The bifunctional enzyme proline utilization A (PutA) catalyzes the two-step oxidation of L-proline to L-glutamate using proline dehydrogenase (PRODH) and L-glutamate-γ-semialdehyde dehydrogenase (GSALDH) domains. The two active sites are 42 Å apart and connected by a buried tunnel that is hypothesized to channel the intermediates Δ1-pyrroline-5-carboxylate (P5C) and/or L-glutamate-γ-semialdehyde (GSAL). The PRODH active site is located in a (βα)8 barrel, while the GSALDH module features Rossmann NAD+-binding and catalytic domains, which are both characteristic of the ALDH superfamily. Kinetic and conventional X-ray crystallography of PutA from Sinorhizobium meliloti (SmPutA) were used to capture high resolution (1.47–1.88 Å) structures of states along the catalytic cycle, including a novel FADH−-proline covalent adduct in the PRODH site, the intermediate P5C bound noncovalently in the reduced PRODH active site, the covalent acyl-enzyme intermediate of the GSALDH reaction, and noncovalent complexes of GSAL and the final product L-glutamate in the GSALDH active site.

The structure of SmPutA complexed with the product L-glutamate was determined at 1.50 Å resolution. The complex was prepared by soaking WT crystals with 325 mM L-glutamate. Electron density for the product is strong in both chains in the asymmetric unit, enabling modeling of the ligand at occupancy of 1.0. L-glutamate adopts an extended conformation, with its backbone interacting with the anchor loop, the side chain carboxylate in the oxyanion hole, and the aliphatic chain in the aromatic box. Cys844 in this complex exhibits χ1 of −69°, instead of the nucleophilic attack rotamer (55°), to avoid steric clash with the side chain carboxylate of the product. The interactions of the product are similar to those of GSAL in the noncovalent complex and the acyl-enzyme intermediate. Although we have focused on the enzyme-ligand complexes, the glutamate complex structure also reveals the conformation of the ligand-free, oxidized PRODH active site, which potentially provides information about conformational changes associated with the binding of proline. The conformational change of Tyr485 is striking, with the hydroxyl group of the side chain moving 14 Å. Conformational differences in the FAD are also evident and imply a crankshaft rotation of the ribityl chain upon proline binding to the resting enzyme.

>[2x]SMMSPNPLQKPAIDAAPAPFADFAPPVRPQSTLRRAITAAYRRPETECLPPLVEAATQSKEIRDAAASTARKLIEALRGKHSGSGVEGLVQEYSLSSQEGVALMCLAEALLRIPDTATRDALIRDKIADGNWKSHLGGSRSLFVNAATWGLVVTGKLTSTVNDRSLAAALTRLISRCGEPVIRRGVDMAMRMMGEQFVTGETIREALKRSKELEEKGFSYSYDMLGEAATTAADAERYYRDYESAIHAIGKASAGRGIYEGPGISIKLSALHPRYSRAQAARVMGELLPRVKALALLAKNYDIGLNIDAEEADRLELSLDLLEVLCLDGDLSGWNGMGFVVQAYGKRCPFVLDFIIDLARRSGRRIMVRLVKGAYWDAEIKRAQLDGLADFPVFTRKIHTDVSYIACAAKLLAATDVVFPQFATHNAQTLAAIYHMAGKDFHVGKYEFQCLHGMGEPLYEEVVGRGKLDRPCRIYAPVGTHETLLAYLVRRLLENGANSSFVHRINDPKVSIDELIADPVEVVRAMPVVGAKHDRIALPAELFGDARTNSAGLDLSNEETLASLTEALRESAAMKWTALPQLATGPAAGETRTVLNPGDHRDVVGSVTETSEEDARRAVRLAADAAPDWAAVPPSERAACLDRAAELMQARMPTLLGLIIREAGKSALNAIAEVREAIDFLRYYAEQTRRTLGPGHGPLGPIVCISPWNFPLAIFTGQIAAALVAGNPVLAKPAEETPLIAAEGVRILREAGIPASALQLLPGDGRVGAALVAAAETAGVMFTGSTEVARLIQAQLADRLSPAGRPIPLIAETGGQNAMIVDSSALAEQVVGDVITSAFDSAGQRCSALRVLCLQEDVADRILTMLKGALHELHIGRTDRLSVDVGPVITSEAKDNIEKHIERMRGLGRKVEQIGLASETGVGTFVPPTIIELEKLSDLQREVFGPVLHVIRYRRDDLDRLVDDVNATGYGLTFGLHTRLDETIAHVTSRIKAGNLYINRNIIGAVVGVQPFGGRGLSGTGPKAGGPLYLGRLVTTAPVPPQHSSVHTDPVLLDFAKWLDGKGARAEAEAARNAGSSSALGLDLELPGPVGERNLYTLHARGRILLVPATESGLYHQLAAALATGNSVAIDAASGLQASLKNLPQTVGLRVSWSKDWAADGPFAGALVEGDAERIRAVNKAIAALPGPLLLVQAASSGEIARNPDAYCLNWLVEEVSASINTAAAGGNASLMAIG> MSNLSGTDKSVILLMTIGEDRAAEVFKHLSTREVQALSTAMANVRQISNKQLTDVLSEFEQEAEQFAALNINANEYLRSVLVKALGEERASSLLEDILETRDTTSGIETLNFMEPQSAADLIRDEHPQIIATILVHLKRSQAADILALFDERLRHDVMLRIATFGGVQPAALAELTEVLNGLLDGQNLKRSKMGGVRTAAEIINLMKTQQEEAVITAVREFDGELAQKIIDEMFLFENLVDVDDRSIQRLLQEVDS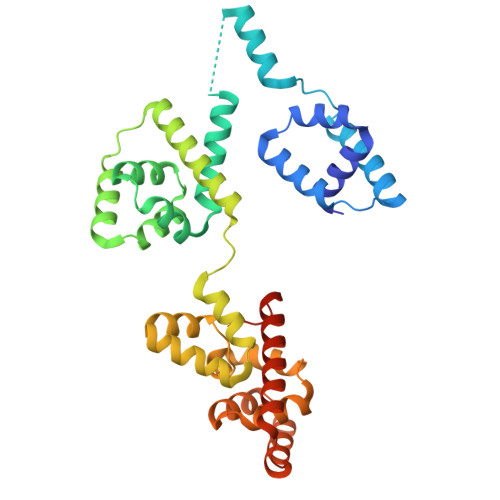ESLLIALKGAEPPLREKFLRNMSQRAADILRDDLANRGPVRLSQVENEQKAILLIVRRLAETGEMVIGSGEDTYV> TELKIGN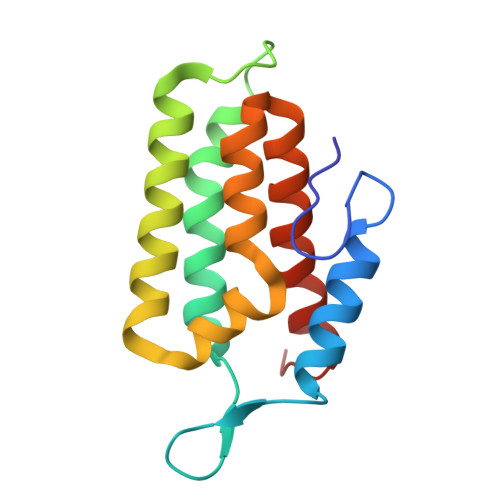EKVNSTNFGDFAEKAIRGINHKPFVNSKGGEQKITTSKIRGILELVNKVYNRVINTNDVELSENILADIAYIKVKIAYESGREPVVKDFIQRTAFTAAITDVMNQRTRESFLLFARYVESLIAYFKFYGGKD>[18x]XGELAQSIKELAKSIK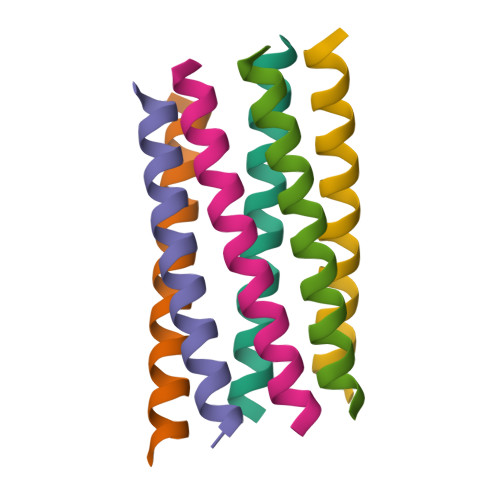ELAWSIKELAQSIKGX> MGHHHHHHMSEFYKLAPVDKKGQPFPFDQLKGKVVLIVNVASKCGFTPQYKELEALYKRYKDE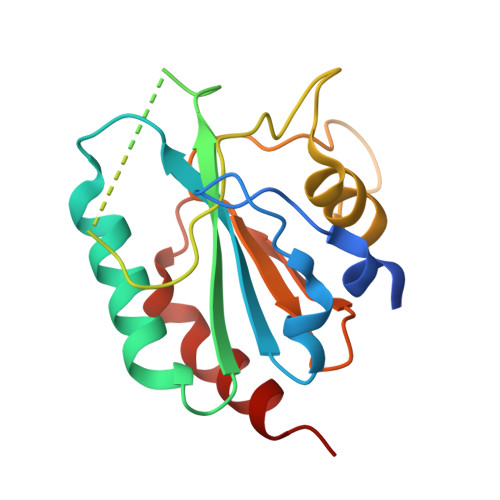GFTIIGFPCNQFGHQEPGSDEEIAQFCQLNYGVTFPIMKKIDVNGGNEDPVYKFLKSQKSGMLGLRGIKWNFEKFLVDKKGKVYERYSSLTKPSSLSETIEELLKEVE>MGSSHHHHHHSSGRENLYFQGMGRVLDRIEVVAEEIRGQAVQSEADCRLTDAAAGLLRDSGAIRLLQPRLYGGYEVHPREFAETVMGVAALDGASGWVTGIVGVHPWELAFADPQVQEEIWGEDNDTWMASPYAPMGVATPVDGGYVLKGRWSFSSGTDHCQWAFLGAMVGDGEGGIATPSSLHVILPRTDYQIVEDTWDVIGLRGTGSKDLIVDGAFVPGYRTLNAAKVMDGRAQKEAGRPEPLFNMPYSCMFPLGITAAVIGITEGALACHIAVQKDRVAITGQKIKEDPYVLSAIGESAAEINASRVSLIETADRFYDKVDAGKEITFEERAIGRRTQIAAAWRAVRAADEIFARAGGGALHYKTPMQRFWRDAHAG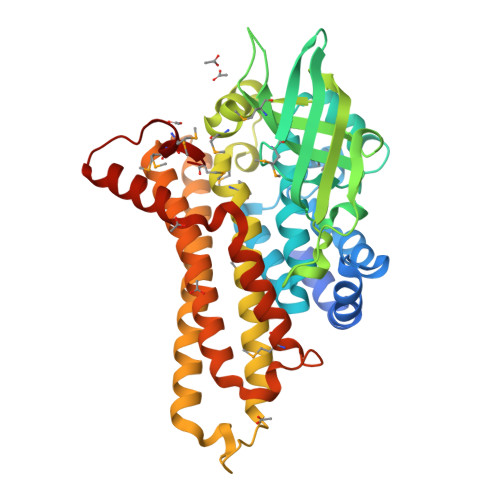LAHAVHVPGPTNHASALTQLGGEPQGMMRAMIGS[2x]> MAHHHHHHVDDDDKMVHHDGFQTVKATIDWEHPMFKLYEKAKRNGKWNPADIDFSQDQKDFASLTSEEKISALPLVAGFSAGEEAVTLDILPMAHALARQGRLEDVLFLTTFMHDEAKHVEMFSRWQQAVGIGQMDLSVFHNDHYKRIFYEALPEAMNRLYADDSPEAVIRAATVYNMIVEGTLAESGYYTFRQIYKKAGLFPGLLQGIDYLNMDEGRHIQFGIYTIQRIVNEDERYYELFIRY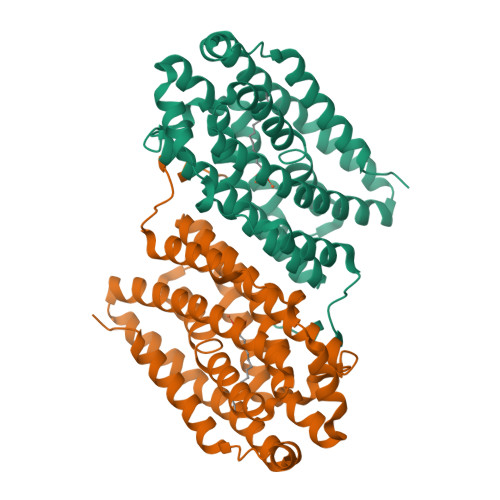MDELWPHVIGYVDYLTELGKRQQQLARTYALEIDYDLLRHYVIKQFNLRKKQISRTKRVDVVEGLEKTAAES> MASVKLTELLDLYREDRGAKWVTALEEIPSLIIKGLSYLQLKNTKQDSLGQLVDWTMQALNLQVALRQPIALNVRQLKAGTKLVSSLAECGAQGVTGLLQAGVISGLFELLFADHVSSSLKLNAFKALDSVISMTEGMEAFLRGRQNEKSGYQKLLELILLDQTVRVVTAGSAILQKCHFYEVLSEIKRLGDHLAEKTSSLPNHSEPDHDTDAGLERTNPEYENEVEASMDMDLLESSNISEGEIERLINLLEEVFHLMETAPHTMIQQPVKSFPTMARITGPPERDDPYPVLFRYLHSHHFLELVTLLLSIPVTSAHPGVLQATKDVLKFLAQSQKGLLFFMSEYEATNLLIRALCHFYDQDEEEGLQSDGVIDDAFALWLQDSTQTLQCITELFSHFQRCTASEETDHSDLLGTLHNLYLITFNPVGRSAVGHVFSLEKNLQSLITLMEYYSKEALGDSKSKKSVAYNYACILILVVVQSSSDVQMLEQHAASLLKLCKADENNAKLQELGKWLEPLKNLRFEINCIPNLIEYVKQNIDNLMTPEGVGLTTALRVLCNVACPPPPVEGQQKDLKWNLAVIQLFSAEGMDTFIRVLQKLNSILTQPWRLHVNMGTTLHRVTTISMARCTLTLLKTMLTELLRGGSFEFKDMRVPSALVTLHMLLCSIPLSGRLDSDEQKIQNDIIDILLTFTQGVNEKLTISEETLANNTWSLMLKEVLSSILKVPEGFFSGLILLSELLPLPLPMQTTQVIEPHDISVALNTRKLWSMHLHVQAKLLQEIVRSFSGTTCQPIQHMLRRICVQLCDLASPTALLIMRTVLDLIVEDLQSTSEDKEKQYTSQTTRLLALLDALASHKACKLAILHLINGTIKGDERYAEIFQDLLALVRSPGDSVIRQQCVEYVTSILQSLCDQDIALILPSSSEGSISELEQLSNSLPN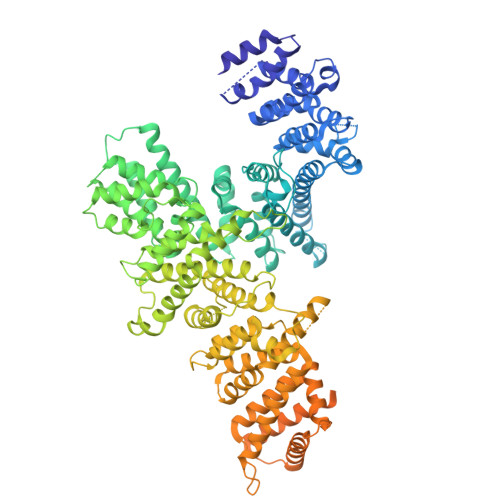KELMTSICDCLLATLANSESSYNCLLTCVRTMMFLAEHDYGLFHLKSSLRKNSSALHSLLKRVVSTFSKDTGELASSFLEFMRQILNSDTIGCCGDDNGLMEVEGAHTSRTMSINAAELKQLLQSKEESPENLFLELEKLVLEHSKDDDNLDSLLDSVVGLKQMLES>[12x]MAEKRTGLAEDGAKSVYERLKNDRAPYETRAQNCAQYTIPSLFPKDSDNASTDYQTPWQAVGARGLNNLASKLMLALFPMQTWMRLTISEYEAKQLLSDPDGLAKVDEGLSMVERIIMNYIESNSYRVTLFEALKQLVVAGNVLLYLPEPEGSNYNPMKLYRLSSYVVQRDAFGNVLQMVTRDQIAFGALPEDIRKAVEGQGGEKKADETIDVYTHIYLDEDSGEYLRYEEVEGMEVQGSDGTYPK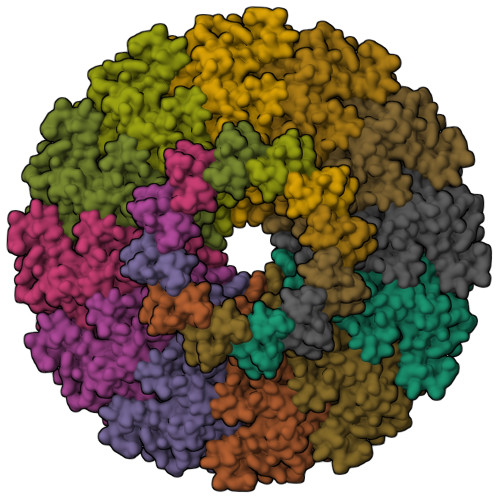EACPYIPIRMVRLDGESYGRSYIEEYLGDLRSLENLQEAIVKMSMISSKVIGLVNPAGITQPRRLTKAQTGDFVTGRPEDISFLQLEKQADFTVAKAVSDAIEARLSFAFMLNSAVQRTGERVTAEEIRYVASELEDTLGGVYSILSQELQLPLVRVLLKQLQATQQIPELPKEAVEPTISTGLEAIGRGQDLDKLERCVTAWAALAPMRDDPDINLAMIKLRIANAIGIDTSGILLTEEQKQQKMAQQSMQMGMDNGAAALAQGMAAQATASPEAMAAAADSVGLQPGI>[4x]AAVILESIFLKRSQQKKKTSPLNFKKRLFLLTVHKLSYYEYDFERGRRGSKKGSIDVEKITCVETVVPEKNPPPERQIPR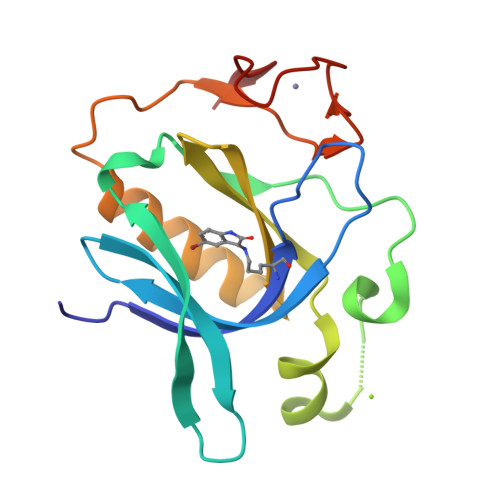RGEESSEMEQISIIERFPYPFQVVYDEGPLYVFSPTEELRKRWIHQLKNVIRYNSDLVQKYHPAFWIDGQYLCCSQTAKNAMGCQILEN> MKVWLVGAYGIVSTTAMVGARAIERGIAPKIGLVSELPHFEGIEKYAPFSFEFGGHEIRLLSNAYEAAKEHWELNRHFDREILEAVKSDLEGIVARKGTALNCGSGIKELGDIKTLEGEGLSLAEMVSRIEEDIKSFADDETVVINVASTEPLPNYS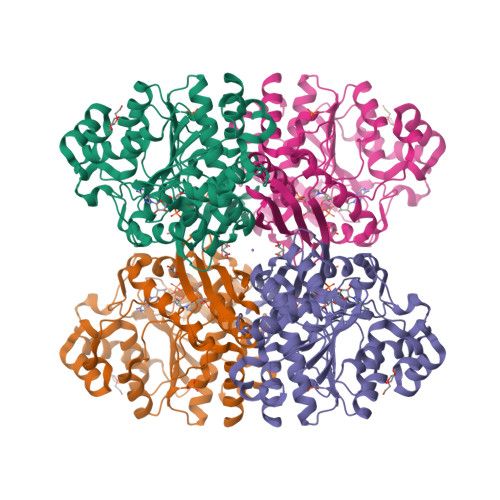EEYHGSLEGFERMIDEDRKEYASASMLYAYAALKLGLPYANFTPSPGSAIPALKELAEKKGVPHAGNDGKTGETLVKTTLAPMFAYRNMEVVGWMSYNILGDYDGKVLSARDNKESKVLSADKVLEKMLGYSPYSITEIQYFPSLVDNKTAFDFVHFKGFLGKLMKFYFIWDAIDAIVAAPLILDIARFLLFAKKKGVKGVVKEMAFFFKSPMDTNVINTHEQFVVLKEWYSNLK> LCLSQQFKAQGDYILGGLFPLGSTEEATLNQRTQPNSIPCNRFSPLGLFLAMAMKMAVEEINNGSALLPGLRLGYDLFDTCSEPVVTMKSSLMFLAKVGSQSIAAYCNYTQYQPRVLAVIGPHSSELALITGKFFSFFLMPQVSYSASMDRLSDRETFPSFFRTVPSDRVQLQAVVTLLQNFSWNWVAALGSDDDYGREGLSIFSSLANARGICIAHEGLVPQHDTSGQQLGKVLDVLRQVNQSKVQVVVLFASARAVYSLFSYSIHHGLSPKVWVASESWLTSDLVMTLPNIARVGTVLGFLQRGALLPEFSHYVETHLALAADPAFCASLNAELDLEEHVMGQRCPRCDDIMLQNLSSGLLQNLSAGQLHHQIFATYAAVYSVAQALHNTLQCNVSHCHVSEHVLPWQLLENMYNMSFHARDLTLQFDAEGNVDMEYDLKMWVWQSPTPVLHTVGTFNGTLQLQQSKMYWPGNQVPVSQCSRQCKDGQVRRVKGFHSCCYDCVDCKAGSYR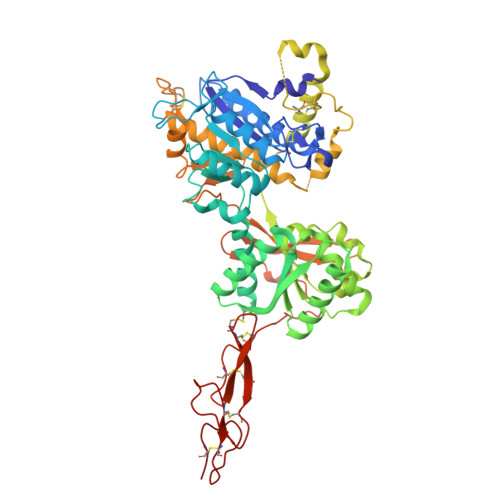KHPDDFTCTPCNQDQWSPEKSTACLP>MKTHILLARVLACAALVLVTPGYSSEKIPVTGSGFVAKDDSLRTFFDAMALQLKEPVIVSKMAARKKITGNFEFHDPNALLEKLSLQLGLIWYFDGQAIYIYDASEMRNAVVSLRNVSLNEFNNFLKRSGLYNKNYPLRGDNRKGTFYVSGPPVYVDMVVNAATMMDKQNDGIELGRQKIGVMRLNNTFVGDRTYNLRDQKMVIPGIATAIERLLQGEEQPLGNIVSSEPPAMPAFSANGEKGKAANYAGGMSLQEALKQNAAAGNIKIVAYPDTNSLLVKGTAEQVHFIEMLVKALDVAKRHVELSLWIVDLNKSDLERLGTSWSGSITIGDKLGVSLNQSSISTLDGSRFIAAVNALEEKKQATVVSRPVLLTQENVPAIFDNNRTFYTKLIGERNVALEHVTYGTMIRVLPRFSADGQIEMSLDIEDGNDKTPQSDTTTSVDALPEVGRTLISTIARVPHGKSLLVGGYTRDANTDTVQSIPFLGKLPLIGSLFRYSSKNKSNVVRVFMIEPKEIVDPLTPDASESVNNILKQSGAWSGDDKLQKWVRVYLDRGQEAIK[15x]

The injectisome is a specialized bacterial organelle that utilizes a type III secretion system (T3SS) to translocate effector proteins from the bacterial cytosol directly into a eukaryotic host. Composed of >20 different proteins, the injectisome forms a syringe shaped nanomachine that spans both bacterial membranes and that of the infected host. The major structural unit of the injectisome is the basal body, composed of three highly oligomerized concentric rings spanning the bacterial inner membrane (IM) (PrgH and PrgK in the Salmonella enterica serovar Typhimurium SPI-1 T3SS)3–6 and outer membrane (OM)7 (InvG, a member of the secretin family of OM pores also found in the type II secretion system, type IV pili system, as well as the phage assembly system). To address this and further elucidate the structural basis for injectisome assembly and function, including that of the central needle component, we have conducted here a cryo-EM analysis of the assembled native needle complex resulting in 3D reconstructions of the IM and OM rings at resolutions permitting atomic model building (3.6 Å and 3.9 Å, respectively) and the 3D reconstruction of an isolated helical needle filament at 3.3 Å resolution.

Although the more peripheral N-terminal N0 and N1 domains were of lower local resolution, the map was of sufficient quality to reveal secondary structure elements for the N1 domain in particular allowing us to position 15 copies of our prior InvG34–173 crystal structure for that domain (PDB 4G085) further expanding the defined model of the injectisome. The final secretin model spanning all domains (residues 34–557, N3 domain loop 228–251 disordered) was refined with density restrained symmetry refinement in Rosetta and notably reveals the dramatic conformational changes involved in secretin gate opening during needle assembly, a fundamental and functionally critical aspect of this giant gated pore family. Overlay of the needle complex and prior closed basal body reconstructions illustrates that the primary sites of conformational change upon needle assembly are in the conserved core secretin region: the N3 ring domain—the tightly oligomerized foundation upon which the secretin assembles7—and the inner β-barrel and membrane associating lip of the central secretin domain, all of which have reoriented to accommodate the presence of the needle filament. The N-terminal N0 and N1 domains, outer β-barrel and C-terminal surface exposed S domain conversely show very little structural difference between assembly states; as with the static IM ring components they appear to provide a highly stable scaffold or shell to buttress the inner conformational changes required for needle passage.>[2x]GSVLQKEGIEISEGTGYDLSKEPGAATVKALEQGTIVISYKTTSENAIQSLLSVGNGTKGNQDRHFHLYITNAGGVGMELRNTDGEFKYTLDCPAAVRGSYKGERVSNTVALKADKENKQYKLFANGELIATLDQEAFKFISDITGVDNVMLGGTMRQGTVAYPFGGSIERMQVYRDVLSDDELIAVTGI

Ruminococcus gnavus is a human gut symbiont wherein the ability to degrade mucins is mediated by an intramolecular trans-sialidase (RgNanH). RgNanH comprises a GH33 catalytic domain and a sialic acid-binding carbohydrate-binding module (CBM40). RgCBM40 displays the canonical CBM40 β-sandwich fold and broad specificity towards sialoglycans with millimolar binding affinity towards α2,3- or α2,6-sialyllactose. RgCBM40 binds to mucus produced by goblet cells and to purified mucins, providing direct evidence for a CBM40 as a novel bacterial mucus adhesin.

Protein ligand complexes were achieved for both 3′SL and 6′SL. Definitive electron density for the Neu5Ac and galactose residues was observed in the 3′SL and 6′SL complexes. Contrastingly, for the 3′SL complex, only partial electron density was observed for the glucose residue in a single monomer, and the glucose positioning indicates that the lactose points up and away from the binding site, without further interactions with the protein. In the 3′SL complex, the lactose positioning would permit further extensions to the carbohydrate chain as would be present in more complex or anchored glycans, whereas these may be blocked in the 6′SL complex. This would provide a degree of specificity towards sialic acid linkage. Notably, the carboxylic acid group of Neu5Ac forms electrostatic interactions with an arginine dyad, Arg204 and Arg128, mimicking the coordination observed in sialidase active sites. The C4 hydroxyl group hydrogen bonds to Lys135 and Glu126, the N-acetyl group sits in a hydrophobic pocket formed by Tyr116 and Ile95. The N-acetyl group nitrogen interacts with both Glu126 and Tyr210. The affinity of the interaction between RgCBM40 and sialic acid ligands was further assessed by ITC. Both 3′SL and 6′SL bound with similar low affinities, with dissociation constants of 0.57 mM and 1.70 mM, respectively.>[2x]MGSSHHHHHHQQKLTSPDNNLVMTFQVDSKGAPTYELTYKNKVVIKPSTLGLELKKEDNTRTDFDWVDRRDLTKLDSKTNLYDGFEVKDTQTATFDETWQPVWGEEKEIRNHYNELAVTLYQPMNDRSIVIRFRLFNDGLGFRYEFPQQKSLNYFVIKEEHSQFGMNGDHIAFWIPGDYDTQEYDYTISRLSEIRGLMKEAITPNSSQTPFSQTGVQTALMMKTDDGLYINLHEAALVDYSCMHLNLDDKNMVFESWLTPDAKGDKGYMQTPCNTPWRTIIVSDDARNILASRITLNLNEPCKIADAASWVKPVKYIGVWWDMITGKGSWAYTDELTSVKLGETDYSKTKPNGKHSANTANVKRY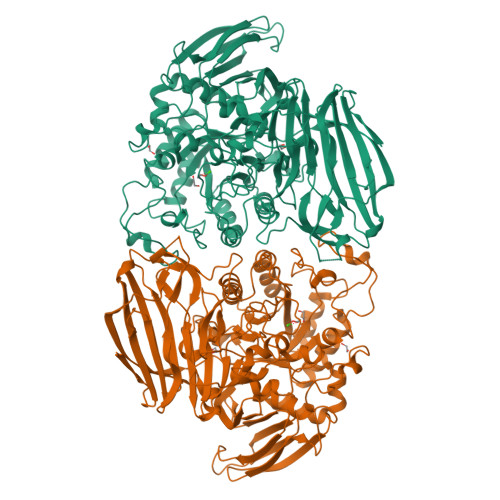IDFAAAHGFDAVLVEGWNEGWEDWFGNSKDYVFDFVTPYPDFDVKEIHRYAARKGIKMMMHHETSASVRNYERHMDKAYQFMADNGYNSVKSGYVGNIIPRGEHHYGQWMNNHYLYAVKKAADYKIMVNAHEATRPTGICRTYPNLIGNESARGTEYESFGGNKVYHTTILPFTRLVGGPMDYTPGIFETHCNKMNPANNSQVRSTIARQLALYVTMYSPLQMAADIPENYERFMDAFQFIKDVALDWDETNYLEAEPGEYITIARKAKDTDDWYVGCTAGENGHTSKLVFDFLTPGKQYIATVYADAKDADWKENPQAYTIKKGILTNKSKLNLHAANGGGYAISIKEVKDKSEAKGLKRL>[2x]MSDKTKTNEGFSRRSFIGSAAVVTAGVAGLGAIDAASATQKTNRASTVKGGFDYDVVVVGGGFAGATAARECGLQGYRTLLLEARSRLGGRTFTSRFAGQEIEFGGAWVHWLQPHVWAEMQRYGLGVVEDPLTNLDKTLIMYNDGSVESISPDEFGKNIRIAFEKLCHDAWEVFPRPHEPMFTERARELDKSSVLDRIKTLGLSRLQQAQINSYMALYAGETTDKFGLPGVLKLF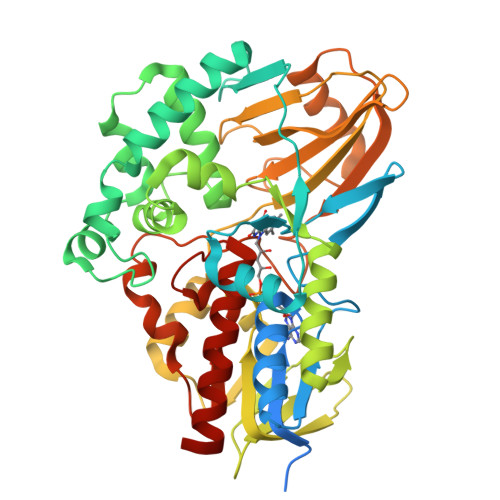ACGGWNYDAFMDTETHYRIQGGTIGLINAMLTDSGAEVRMSVPVTAVEQVNGGVKIKTDDDEIITAGVVVMTVPLNTYKHIGFTPALSKGKQRFIKEGQLSKGAKLYVHVKQNLGRVFAFADEQQPLNWVQTHDYSDELGTILSITIARKETIDVNDRDAVTREVQKMFPGVEVLGTAAYDWTADPFSLGAWAAYGVGQLSRLKDLQAAEGRILFAGAETSNGWHANIDGAVESGLRAGREVKQLLSLEHHHHHH> MRYKFLSEQKEDLTEAKNTLFQVIEEMDEEMTKRFNDTFVQIRSHFDQVFRSLFGGGRAELRLT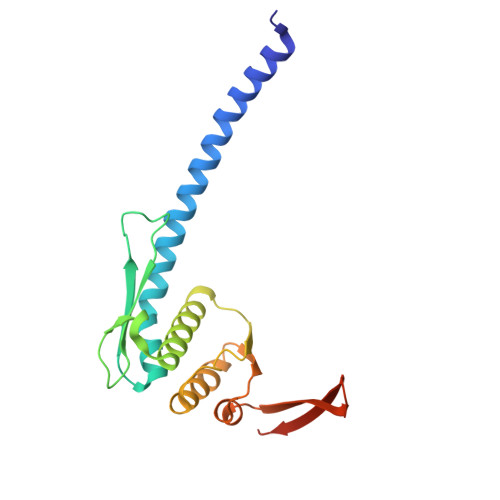DPNDLLHSGVEIIAQPPGKKLQNLNLLSGGERALTAIALLFSILKVRPVPFCVLDQVEAALDEANVFRFAQYLKKYSSDTQFIVITHRKGTMEEADVLYGVTMQESGVSKVISVKLEETKEFVQ ETHYL 4-[(4-CHLOROPYRIDIN-2-YL)AMINO]PIPERIDINE-1-CARBOXYLATE 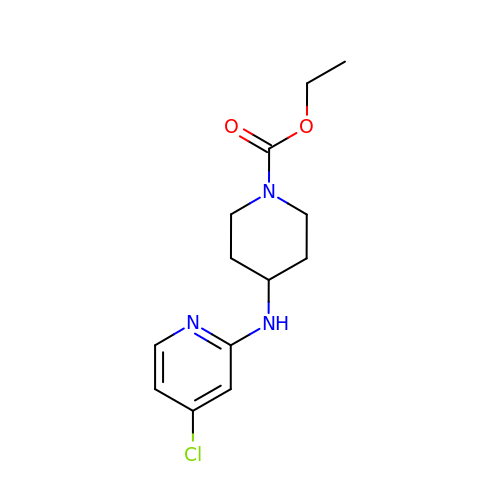| C13 H18 Cl N3 O2 | YQEYLCGMINXDBN-UHFFFAOYSA-N> MLRRALLCLAVAALVRADAPEEEDHVLVLRKSNFAEALAAHKYLLVEFYAPWCGHCKALAPEYAKAAGKLKAEGSEIRLAKVDATEESDLAQQYGVRGYPTIKFFRNGDTASPKEYTAGREADDIVNWLKKRTGPAATTLPDGAAAESLVESSEVAVIGFFKDVESDSAKQFLQAAEAIDDIPFGITSNSDVFSKYQLDKDGVVLFKKFDEGRNNFEGEVTKENLLDFIKHNQL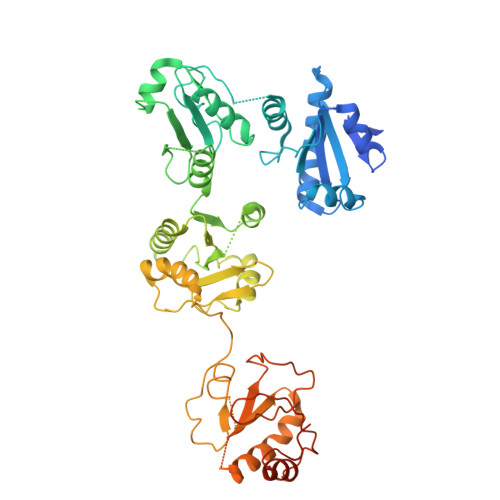PLVIEFTEQTAPKIFGGEIKTHILLFLPKSVSDYDGKLSNFKTAAESFKGKILFIFIDSDHTDNQRILEFFGLKKEECPAVRLITLEEEMTKYKPESEELTAERITEFCHRFLEGKIKPHLMSQELPEDWDKQPVKVLVGKNFEDVAFDEKKNVFVEFYAPWCGHCKQLAPIWDKLGETYKDHENIVIAKMDSTANEVEAVKVHSFPTLKFFPASADRTVIDYNGERTLDGFKKFLESGGQDGAGDDDDLEDLEEAEEPDMEEDDDQKAVKDEL>RYNDYKLDFRRQQMQDFFLAHKDEEWFRSKYHPDEVGKRRQEARGALQNRLRVFLSLMETGWFDNLLLDIDKADAIVKMLDAAVIKMEGGTENDLRILEQ[2x];>GLECKPRPLHKTCSLFMRNIAPNISRAEIISLCKRYPGFMRVALSEPQPERRFFRRGWVTFDRSVNIKEICWNLQNIRLRECELSPGVNRDLTRRVRNINGITQHKQIVRNDIKLAAKLIHTLDDRTQLWASEPGTPPLPTSLPSQNPILKNITDYLIEEVSAEEEELLGSSGGAPPEEPPKEGNPAEINVERDEKLIKVLDKLLLYLRIVHSLDYYNTCEYPNEDEMPNRCGIIHVRGPMPPNRISHGEVLEWQKTFEEKLTPLLSVRESLSEEEAQKMGRKDPEQEVEKFVTSNTQELGKDKWLCPLSGKKFKGPEFVRKHIFNKHAEKIEEVKKEVAFFNNFLTDAKRPALPE[2x]

ARS2 is a direct interaction partner of CBC and together they form a platform for the assembly of co-transcriptional complexes that determine the fate of diverse RNA Pol II transcripts. Our structural analysis shows that ARS2 is made up of two regions, residues 147–270 and 408–763 that co-fold into a structured core with an intervening glutamate-rich region of unknown function that is likely unstructured. The human ARS2 core has an unusual structure comprising a largely helical ‘body’ from which project N- and C-terminal ‘legs’. We find that the RRM domain is required to bind RNA, whereas a basic patch in the C-terminal leg of ARS2 mediates the interaction with FLASH.

Based on the incomplete model, the N-terminal helix was truncated at position 171 with the aim of producing better crystals. ARS2171–270+408–763 crystallised in hexagonal space groups P6522 or P65, diffracting to 3.2 and 3.5 Å resolution, respectively. In mammals, loop A (538-ASEPGT543PPLPTSLPS-552) is highly conserved and proline-rich. In most crystal forms, the loop is disordered presumably due to flexibility. In all crystal structures of hARS2 (except that with loop B deleted), only the first part of the loop is observed with 570-AEEEELL forming helix α10 (‘EEEE helix’). Remarkably, all crystal forms containing loop B, irrespective of space-group, exhibit the same intermolecular crystal contact, in which the acidic ‘EEEE helix’ and the preceding short β-strand pack into the positively charged cradle formed by the RRM β-sheet and the C-terminal extension of the RRM. To accommodate the same intermolecular contact in different crystal-packing environments, some angular flexibility of the loop B structure is required. Concerning loop B, in most ARS2 crystal forms the negatively charged ‘EEEE’ helix binds onto the positively charged RRM β-sheet surface of a neighbouring molecule. Repetition of this inter-molecular contact generates a three-dimensional network.We report here that surface‐expressed β protein of GBS binds to human CEACAM1 and CEACAM5 receptors. Human CEACAMs are a family of 12 cellular receptors belonging to the immunoglobulin (Ig) superfamily (IgSF) that are commonly expressed on epithelial cells, endothelial cells and leucocytes (Gray‐Owen & Blumberg, 2006). β protein is a multifunctional protein and interacts with several proteins of the human immune system, including factor H, Siglec‐5, Siglec‐7, Siglec‐14 and IgA, through distinct domains. A crystal structure of the complex showed that an IgSF domain in β represents a novel Ig‐fold subtype called IgI3, in which unique features allow binding to CEACAM1.

We solved the structure in complex with CEACAM1‐N at a resolution of 3.25 Å. The asymmetric unit contains two molecules of the (β‐IgSF)‐(CEACAM1‐N) complex, which are similar to each other when superimposed (r.m.s.d 0.20 Å). The β‐IgSF domain has two β‐sheets labelled ABED and A′GFC, with sheets connected by the BC, EF, CD and AA′ loops. The unique features of this domain are (a) the absence of cysteine residues, (b) absence of C′ and C′′ strands and (c) a truncated C strand that is directly followed by a 1.5‐turn α‐helix. Specifically, L46 in the α‐helix of β‐IgI3 interacts by van der Waals forces with F29 and L95 (distances 3.34 Å and 3.59 Å) located in the C and G strands of CEACAM1, respectively (Fig EV3D). In addition, the protruding β‐IgI3 residue V53 is within close contact of I91 (distance 3.36 Å, F strand), Q44 (distance 2.50 Å, C to C’ loop) and S32 (distance 3.41 Å, C strand) of CEACAM1, D55 is within close contact of Y34 (distance 3.50 Å, C strand) and G41 (distance 2.90 Å, C to C’ loop) of CEACAM1, and F42 is in close contact of L95 (distance 2.87 Å, G strand) of CEACAM1. No conformational changes were observed in CEACAM1 upon binding of β‐IgI3 (Fig EV3E). For CEACAM1‐N, the crystal structure of the complex indicated that β‐IgI3 interacts with the dimer interface, contacting several residues which are important for CEACAM1 homodimerisation and for binding to other bacterial adhesins. In contrast, β‐IgI3 interacts through the small α helix and loop, with a single residue, L46, critical for β‐IgI3 to fit into a pocket on CEACAM1‐N formed by F29 and I91.

>[2x]MAQLTTESMPFNVAEGKEVLLLVHNLPQQLFGYSWYKGERVDGNRQIVGYAIGTQQATPGPANSGRETIYPNASLLIQNVTQNDTGFYTLQVIKSDLVNEEATGQFHVY;>[2x]ANENNQQKIELTVSPENITVYEGEDVKFTVTAKSDSKTTLDFSDLLTKYNPSVSDRISTNYKTNTDNHKIAEITIKNLKLNESQTVTLKAKDDSGNVVEKTFTITVQKKEEKQLPSTGGSHHHHHH> TYMNNTEAICDVKGFAPFSKDNGIRIGSRGHIFVIREPFVSCSPIECRTFFLTQGSLLNDKHSNGTVKDRSPFRTLMSVKVGQSPNVYQARFEAVAWSATACHDGKKWMTVGVTGPDSKAVAVIHYGGVPTDVINSWAGDILRTQESSCTCIQGDCYWVMTDGPANRQAQYRIYKANQGRIIGQADISFNGGHIEECSCYPNDGKVECVCRDNWTGTNRPVLVISPDLSYRVGYLCAGIPSDTPRGEDAQFTGSCTSPMGNQGYGVKGFGFRQGTDVWMGRTISRTSRSGFEILRIKNGWTQTSKEQVRKQVVVDNLNWSGYSGSFTLPVELSGKDCLVPCFWVEMIRGKPEEKTIWTSSSSIVMCGVDYEIADWSWHDGAILPFDIDKM

The Influenza neuraminidase (NA) surface glycoprotein is responsible for the cleavage of sialic acid residues from the surface of the infected cell. Inhibition of this process prevents the release of nascent virions from the surface of the cell, reducing the spread of the infection. Specifically, in the active sites of group 1 NAs a loop, consisting of residues 147–152 (the 150-loop), adopts a conformation leading to the opening of a pocket to the side of the active site (also known as the 150 cavity). While complexes of N8:4 and N8:5 interact in a manner similar to previous NA inhibitors, the structures of N8:6–8 indicate novel binding modes employing contacts with residues within the 150-loop and cavity.

The parental compound within this class is the Oseltamivir isomer 4, in which the cyclohexene double bond has been moved to the C2–C3 position. To understand the molecular basis behind the inhibitory activity of this novel class of inhibitors, crystal structures of the parental compounds 4 and 5 were obtained in complex with a group-1 NA by soaking crystals of N8 [A/duck/Ukraine/1/63 (H3N8)] enzyme in 1 mM solutions of compound. In both N8:4 and N8:5 complexes, the inhibitors bound in a position and orientation very similar to that observed previously in structures of N8:1. In particular, N8:4 overlays almost exactly with N8:1, with only a subtle repositioning of the C7 atom due to the change in position of the double bond in the cyclohexene ring relative to 1. Surprisingly, given the lower activity of compound 4 in in vitro inhibition assays, no further significant differences in the position of the compound's pendant groups or active site residues were observed. Comparison with N8:4 indicates that these direct hydrogen bonds replace a looser network of water-mediated interactions, with retention of only the direct contact between the amino group of 4 and E119. The structures of the N8:4 and N8:5 complexes are remarkably similar to N8:1, suggesting that the reduced susceptibility of these compounds is not due to substantial changes to the position of the compounds within the active site. Compounds 4 and 5 inhibited the replication of WT with ED50 values similar to, or lower than that achieved by Oseltamivir. While the inhibition of 4 against the H274Y virus was poor (ED50 > 500 μM), the concentration of 5 required was approximately 10-fold higher than for wild-type virus (ED50 = 34 μM compared to ED50 = 3.9 μM).> GLIVDTRDVEERVHVMRKTKLAPTVAHGVFNPEFGPAALSNKDPRLNEGVVLDEVIFSKHKGDTKMSAEDKALFRRCAADYASRL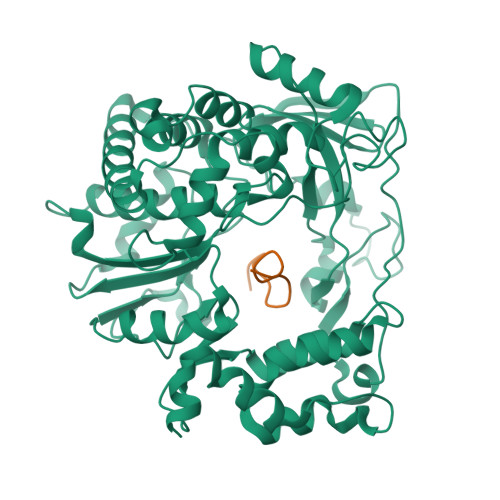HSVLGTANAPLSIYEAIKGVDGLDAMEPDTAPGLPWALQGKRRGALIDFENGTVGPEVEAALKLMEKREYKFACQTFLKDEIRPMEKVRAGKTRIVDVLPVEHILYTRMMIGRFCAQMHSNNGPQIGSAVGCNPDVDWQRFGTHFAQYRNVWDVDYSAFDANHCSDAMNIMFEEVFRTEFGFHPNAEWILKTLVNTEHAYENKRITVEGGMPSGCSATSIINTILNNIYVLYALRRHYEGVELDTYTMISYGDDIVVASDYDLDFEALKPHFKSLGQTITPADKSDKGFVLGHSITDVTFLKRHFHMDYGTGFYKPVMASKTLEAILSFARRGTIQEKLISVAGLAVHSGPDEYRRLFEPFQGLFEIPSYRSLYLRWVNAVCGDAAALE;> GPYAGPLERQRPLKVRAKLPRQE> KLPPGWEKRMSRSSGRVY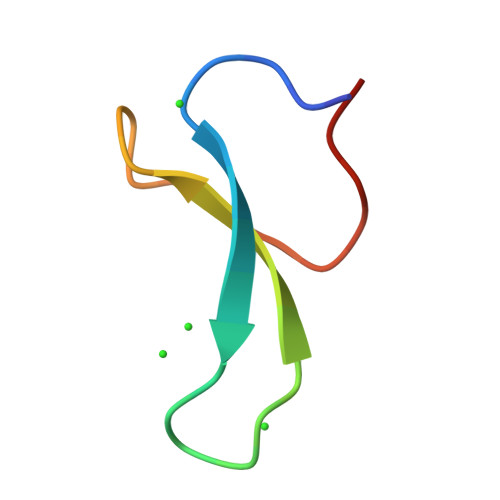YFNHITNASQWERPSG> MERAFQNRCEPRAAKPFKILKKR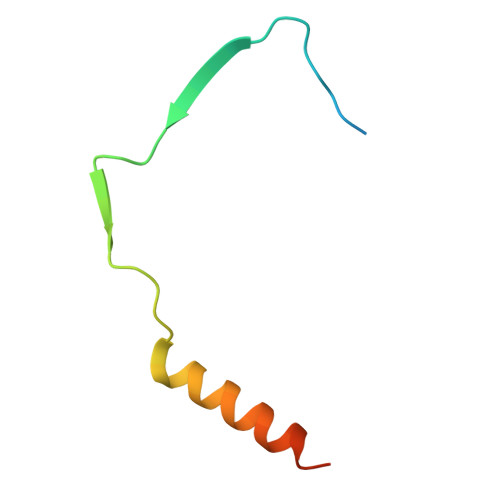STTSVASYQVSPHTARIFKENERLIDEYKRKKA>GHMNKDNLRSPICCILGHVRTGKTKLLDKIRQTNVQEGEAGGITQQIGATYFPVEAIKQKTAVVNKDGKFEFKVPGLLIIDTPGHESFSNLRSRGSSLCNIAILVVDIMHGLEPQTIESLRLLRERKTPFVVALNKIDRLYGWKKIENNGFRESFALQNKAVQNEFRNRLDQVKLQFAEQGFNSELFYENKNFARYVSLVPTSAHTGEGIPDMLKLIVQLCQERMASSLMYLSELQATVLEVKAIEGFGVTIDVILSNGILREGDRIVLCGLEGPIKTNIRALLTPAPMRELRIKGQYIHHKEVKAAQ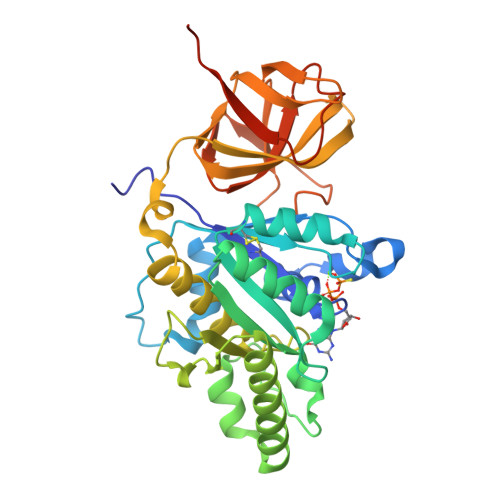GVKISAPGLEGAIAGSRLLVVGPDDDEEELEEEVESD[2x]4-(6,7-dimethoxy-2,4-dihydroindeno[1,2-c]pyrazol-3-yl)phenol 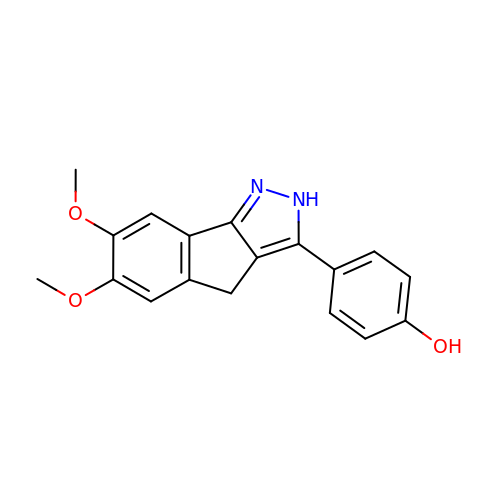| C18 H16 N2 O3 | YXCSLEHSWRLDHG-UHFFFAOYSA-N>[2x]MALRTMVDPDTCTSCELCYDRVPEVYKNRGDGI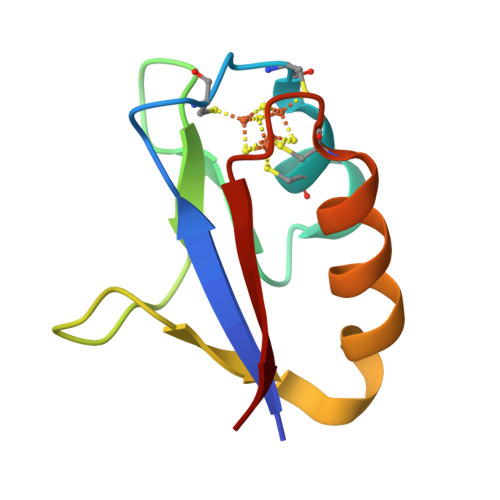AEVVSPGPDGWMMVPPELEQEVKEVTDECPSGSIITEEV>[2x]GPLGSMASKKVCIVGSGNWGSAIAKIVGGNAAQLAQFDPRVTMWVFEEDIGGKKLTEIINTQHENVKYLPGHKLPPNVVAVPDVVQAAEDADILIFVVPHQFIGKICDQLKGHLKANATGISLIKGVDEGPNGLKLISEVIGERLGIPMSVLMGANIASEVADEKFCETTIGCKDPAQGQLLKELMQTPNFRITVVQEVDTVEICGALKNVVAVGA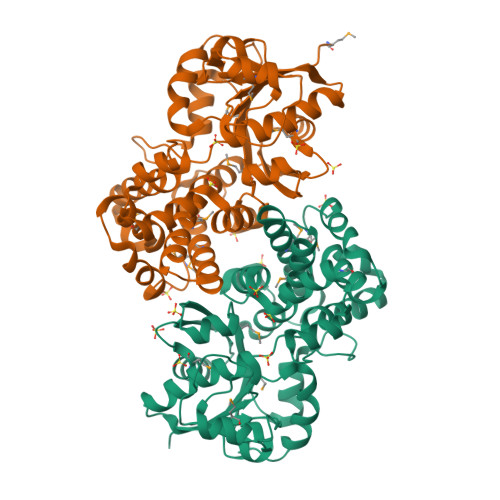GFCDGLGFGDNTKAAVIRLGLMEMIAFAKLFCSGPVSSATFLESCGVADLITTCYGGRNRKVAEAFARTGKSIEQLEKELLNGQKLQGPETARELYSILQHKGLVDKFPLFMAVYKVCYEGQPVGEFIHCLQNHPEHM>[2x]MKTSEQRVNIATLLTENKKKIVDKASQDLWRRHPDLIAPGGIAFSQRDRA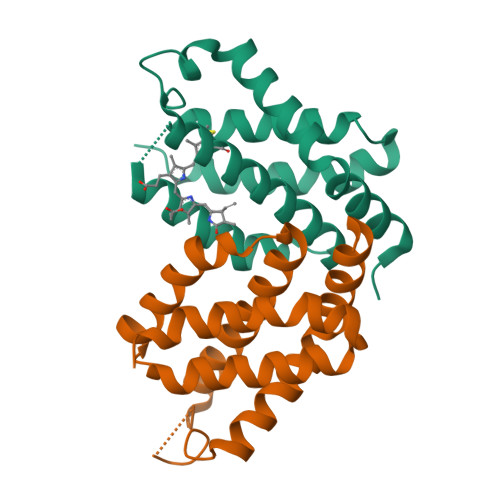LCLRDRGWFLHLITFCLLAGDKGPIESIGLISIREMYNSLGVPVPAMMESIRCLKEASLSLLDEEDANETAPYFDYIIKAMSHHHHHH> AMVHHHHHHSAACPSQCSCSGTTVDCRSKRHASVPAGIPTNAQILYLHDNQITKLEPGVFDSLINLKELYLGSNQLGALPVGVFDSLTQLTVLDLGTNQLTV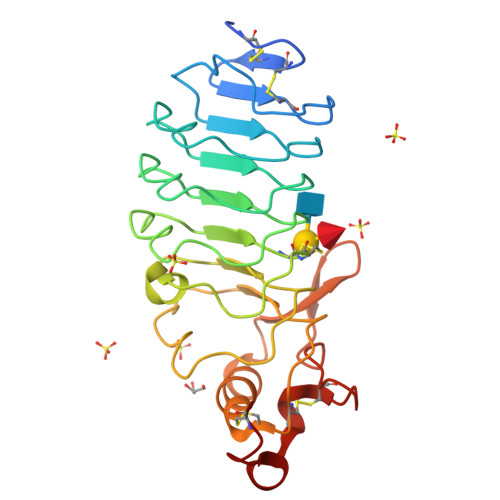LPSAVFDRLVHLKELFMCCNKLTELPRGIERLTHLTHLALDQNQLKSIPHGAFDRLSSLTHAYLFGNPWDCECRDIMYLRNWVADHTSIAMRWDGKAVNDPDSAKCAGTNTPVRAVTEASTSPSKCP> MDWVVAPISVPENGEGPFPQR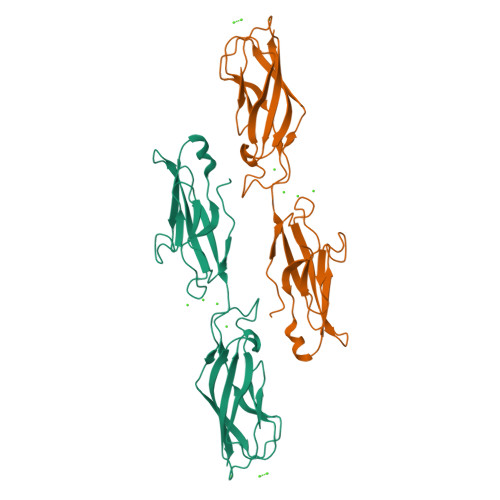LNQLKSNKDRDTKIFYSITGPGADSPPEGVFAVEKETGWLLLNKPLDREEIAKYELFGHAVSENGASVEDPMNISIIVTDQNDHKPKFTQDTFRGSVLEGVLPGTSVMQVTATDEDDAIYTYNGVVAYSIHSQEPKDPHDLMFTIHRSTGTISVISSGLDREKVPEYTLTIQATDMDGDGSTTTAVAVVEILD> MKNIIPQALLTMPILSTGLQAQEKQPTPNLVFIMADQYRGDAIGCIGKEPVKTPHLDKLASEGINFTNAISSYPVSSPARGMLMTGMYPIGSKVTGNCNSETAPYGVELSQNARCWSDVLKDQGYNMGYIGK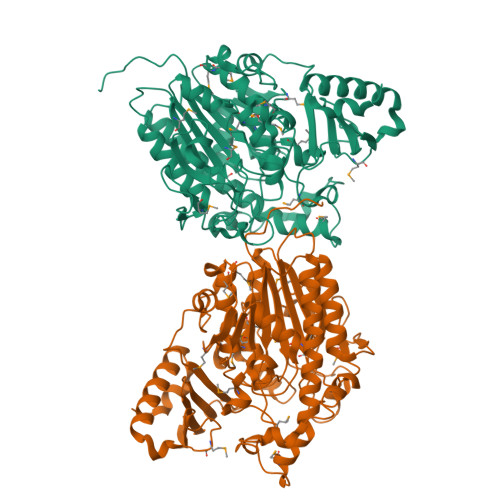WHLDAPYKPYVDTYNNRGKVAWNEWCPPERRHGFDHWIAYGTYDYHLKPMYWNTTAPRDSFYYVNQWGPEYEASKAIEYINGQKDQKQPFALVVSMNPPHTGYELVPDRYKEIYKDLDVEALCKGRPDIPAKGTEMGDYFRNNIRNYYACITGVDENVGRIIEALKQNNLFDNTIVVFTSDHGICMGAHENAGKDIFYEESMRIPMILSWPDQIKPRKSDPLMIAFADLYPTLLSMMGFSKEIPETVQTFDLSNEVLTGKNKKDLVQPYYFVKFDNHATGYRGLRTDRYTYAVHATDGKIDNVILFDRTNDPHEMNNIASQQLKLTHTFNRQLKTWLEKTNDPFAQYIKLKLEHHHHHH> CGCACG;> 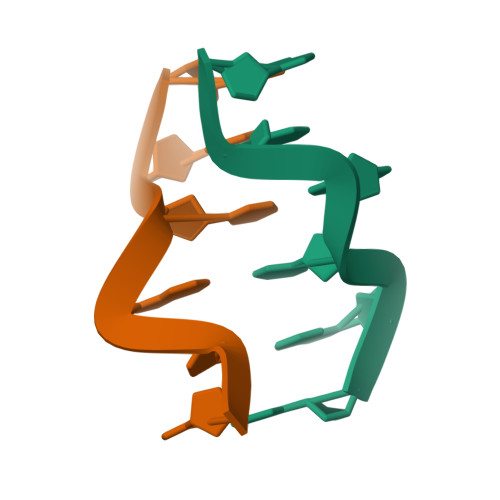CGTGCG> GSSQLPQNIQFSPSAKLQEVLDYLTNSASLQMKSPAITATLEGKNR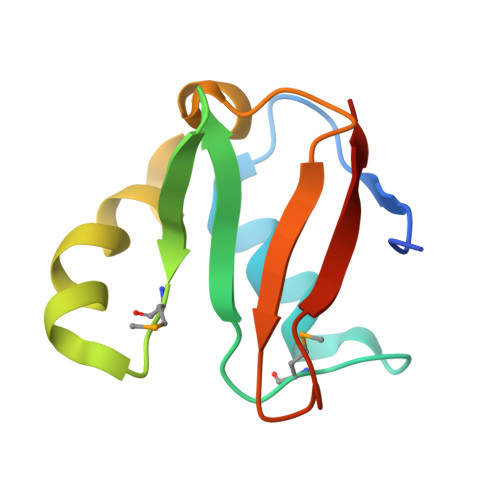TLYMQSVTSIEERTRPNLSKTLKELGLVDGQELAVADVTTPQTVLFKLHFTS>MLNPIVRKFQYGQHTVTLETGMMARQATAAVMVSMDDTAVFVTVVGQKKAKPGQDFFPLTVNYQERTYAAGRIPGSFFRREGRPSEGETLIARLIDRPIRPLFPEGFVNEVQVIATVVSVNPQVNPDIVAMIGASAALSLSGIPFNGPIGAARVGYINDQYVLNPTQDELKESKLDLVVAGTEAAVLMVESEAQLLSEDQMLGAVVFGHEQQQVVIQNINELVKEAGKPRWDWQPEPVNEALNARVAALAEARLSDAYRITDKQERYAQVDVIKSETIATLLAEDETLDENELGEILHAIEKNVVRSRVLAGEPRIDGREKDMIRGLDVRTGVLPRTHGSALFTRGETQALVTATLGTARDAQVLDELMGERTDTFLFHYNFPPYSVGETGMVGSPKRREIGHGRLAKRGVLAVMPDMDKFPYTVRVVSEITESNGSSSMASVCGASLALMDAGVPIKAAVAGIAMGLVKEGDNYVVLSDILGDEDHLGDMDFKVAGSRDGISALQMDIKIEGITKEIMQVALNQAKGARLHILGVMEQAINAPRGDIS[12x];>[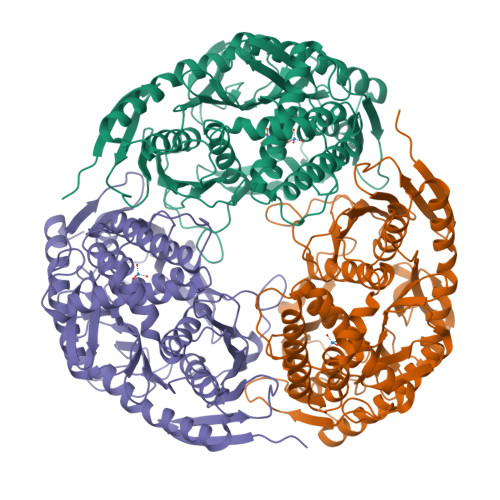12x]EAPRHSDWQRPTFAFEGKGAAGGHTATHHASAAPARPQPVE>MSKPQPIAAANWKCNGSQQSLSELIDLFNSTSINHDVQCVVAPSWYMGAQAMTKERLSHPKFVIAAQNAGNADALASLKDFGISWIVLDHSERRAYYGETNEIVADKVAAAVASGFMVIACIGETLQERSSGRTAVVVLTQITAIAKKLKKADWAKVVIAYEPVWAIGTGKVATPQQAQEAHALIRSW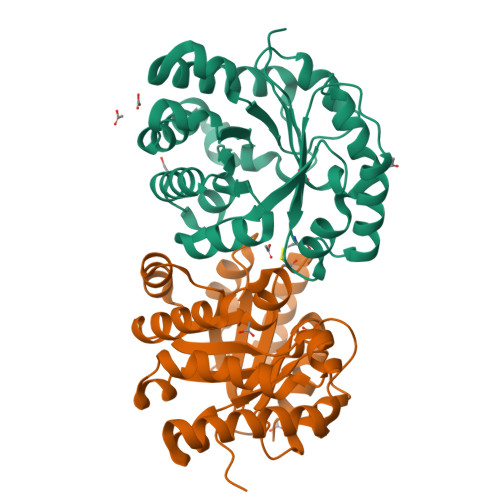VSSKVGADVAGELRILYGGSVNGRNARTLYQQRDVNGFLVGGASLKPEFVDIIKATE[4x]4-methoxy-3-(3-methoxypropoxy)-N-{[(3S,4S)-4-{[(4-methylphenyl)sulfonyl]amino}pyrrolidin-3-yl]methyl}-N-(propan-2-yl)benzamide 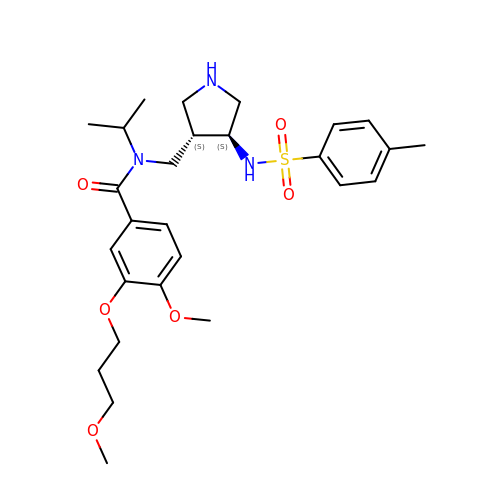| C27 H39 N3 O6 S | RCXREJXZQYBNRM-LADGPHEKSA-N> AIGPVADLKIVNANIQPDGFTRPAVLAGGTFPGPLIKGNKGDNFQLNVIDELENEDMLKSTSIHWHGFFQHGTNWADGPAFVNQCPITTGHSFLYNFHVPDQAGTFWYHSHLSTQYCDGLRGPMVVYDPHDPLKQLYDVDDESTVMTLADWYHTLARQEPPGPVTPDSTLINGLGRAPGQTTPSELAVLTVKRGTRYRIRLINISCEPNYHYSIDNHDLTVIEADGVSTQSLTVSSLTIFAGQRYSFILNANQPVGNYWIRAQPNDAADVTFNGGINSAILRYEGAPVAEPNTTAGPDNTPLLEVNIRPFVFTPVPGQPHAGGADFVKNL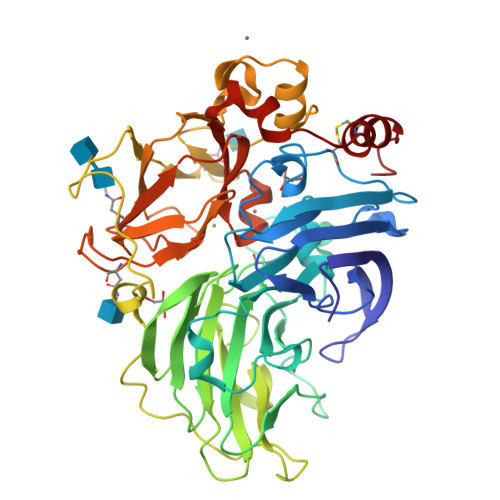LFSFNGTNFQVDNVSFVPPTVPILLQILSGAHTAQDLMPAGSIIPLPKNAVIEFSMPGGVVGGGHPIHLHGHNFWVIRSANSSVYNYNDPVIRDVVNIGTTGDNVTIRFETNNPGPWFLHCHIDWHLDLGFAVVMAEDIPDAAAANPVPAAWNELCPLYDALTPGNQ> MGPHHHHHHLESTSLYKKAGSENLYFQSVAILQKRDHEGFGFVLRGAKAETPIEEFTPTPAFPALQYLESVDVEGVAWKAGLRTGDFLIEVNGVNVVKVGHKQV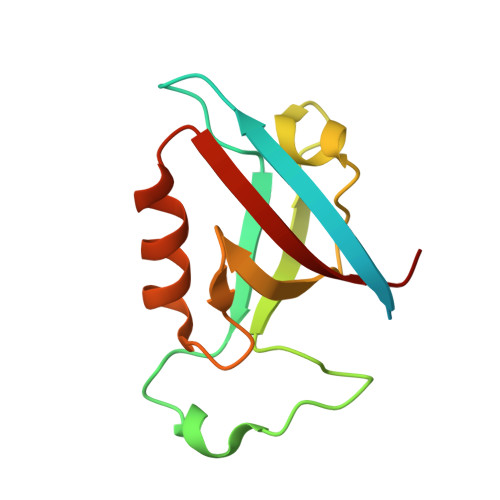VGLIRQGGNRLVMKVVSVT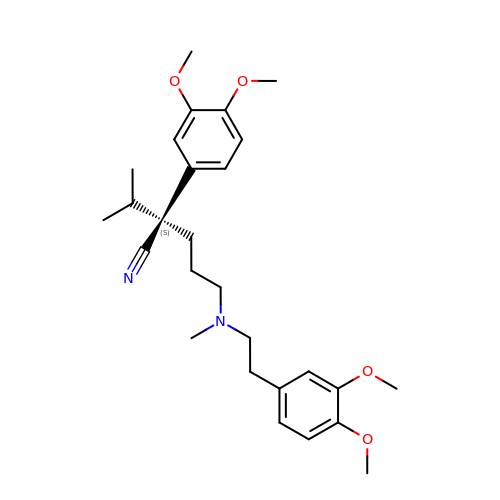(2S)-2-(3,4-dimethoxyphenyl)-5-{[2-(3,4-dimethoxyphenyl)ethyl](methyl)amino}-2-(propan-2-yl)pentanenitrile | C27 H38 N2 O4 | SGTNSNPWRIOYBX-MHZLTWQESA-N>QIANVVLADGQAAPADKTFEPQRGQNGVTDPAEWWEKSSPTLNGYRRLTALVRRNAASKSVKVKVAIYDPTLAVTAPSTASGIQPSPTVAFTCPVFIEFTLPDACTIQNRKDILAYAKNFLASATATDLVVNTAP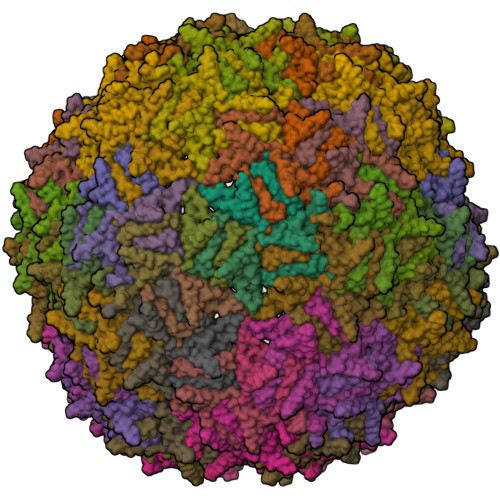QY[60x]HYDROGEN PEROXIDE | H2 O2 | 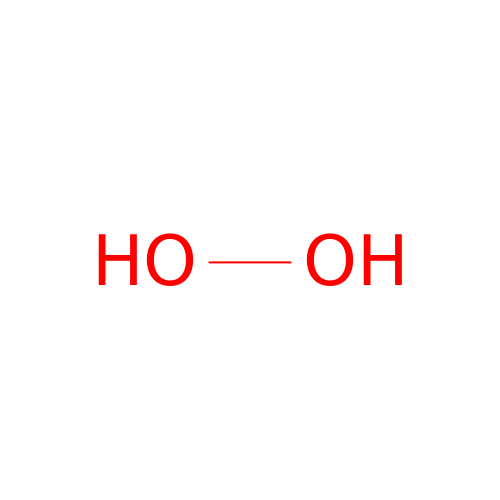MHAJPDPJQMAIIY-UHFFFAOYSA-N> MQYTNKYHEKWIS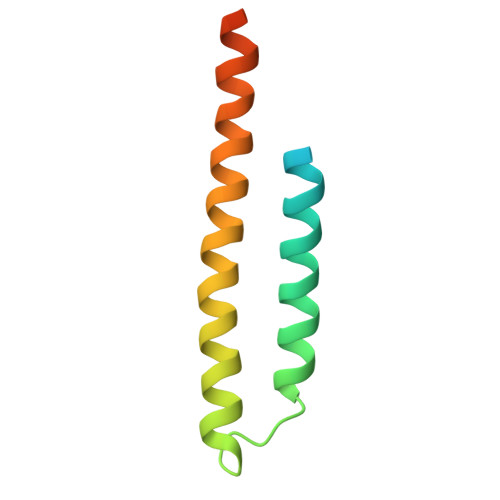KFAPGNELSKKYLAKVKERHELKEFNNSISAQDNYAKWTKNNRKLDSLDKEINNLKDEIQSENKAFQAHLHKLEHHHHHH> GGSGGSMPPPADIVKVAIEWPGAYPKLMEIDQKKPLSAIIKEVCDGWSLANHEYFALQHADSSNFYITEKNRNEIKNGTILRLTTSPAQNAQQLHERIQSSSMDAKLEALKDLASLSRDVTFAQEFINLDGISLLTQMVESGTERYQKLQKIMKPCFGDMLSFTLTAFVELMDHGIVSWDTFSVAFIKKIASFVNKSAIDISILQRSLAILESMVLNSHDLYQKVAQEITIGQLIPHLQGSDQEIQTYTIAVINALFLKAPDERRQEMANIL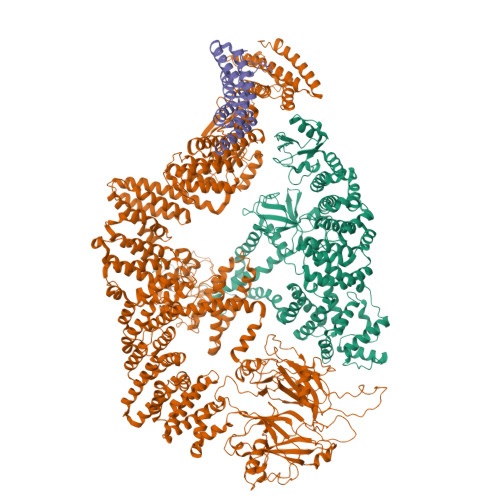AQKQLRSIILTHVIRAQRAINNEMAHQLYVLQVLTFNLLEDRMMTKMDPQDQAQRDIIFELRRIAFDAESEPNNSSGSMEKRKSMYTRDYKKLGFINHVNPAMDFTQTPPGMLALDNMLYFAKHHQDAYIRIVLENSSREDKHECPFGRSSIELTKMLCEILKVGELPSETCNDFHPMFFTHDRSFEEFFCICIQLLNKTWKEMRATSEDFNKVMQVVKEQVMRALTTKPSSLDQFKSKLQNLSYTEILKIRQSERMNQEDFQSRPILELKEKIQPEILELIKQQRLNRLVEGTCFRKLNARRRQDKFWYCRLSPNHKVLHYGDLEESPQGEVPHDSLQDKLPVADIKAVVTGKDCPHMKEKGALKQNKEVLELAFSILYDSNCQLNFIAPDKHEYCIWTDGLNALLGKDMMSDLTRNDLDTLLSMEIKLRLLDLENIQIPDAPPPIPKEPSNYDFVYDCN;>GGSGGSMARWIPTKRQKYGVAIYNYNASQDVELSLQIGDTVHILEMYEGWYRGYTLQNKSKKGIFPETYIHLKEATVEDLGQHETVIPGELPLVQELTSTLREWAVIWRKLYVNNKLTLFRQLQQMTYSLIEWRSQILSGTLPKDELAELKKKVTAKIDHGNRMLGLDLVVRDDNGNILDPDETSTIALFKAHEVASKRIEEKIQEEKSILQNLDLRGQSIFSTIHTYGLYVNFKNFVCNIGEDAELFMALYDPDQSTFISENYLIRWGSNGMPKEIEKLNNLQAVFTDLSSMDLIRPRVSLVCQIVRVGHMELKEGKKHTCGLRRPFGVAVMDITDIIHGKVDDEEKQHFIPFQQIAMETYIRQRQLIMSPLITSHVIGENEPLTSVLNKVIAAKEVNHKGQGLWVSLKLLPGDLTQVQKNFSHLVDRSTAIARKMGFPEIILPGDVRNDIYVTLIHGEFDKGKKKTPKNVEVTMSVHDEEGKLLEKAIHPGAGYEGISEYKSVVYYQVKQPCWYETVKVSIAIEEVTRCHIRFTFRHRSSQETRDKSERAFGVAFVKLMNPDGTTLQDGRHDLVVYKGDNKKMEDAKFYLTLPGTKMEMEEKELQASKNLVTFTPSKDSTKDSFQIATLICSTKLTQNVDLLGLLNWRSNSQNIKHNLKKLMEVDGGEIVKFLQDTLDALFNIMMEMSDSETYDFLVFDALVFIISLIGDIKFQHFNPVLETYIYKHFSATLAYVKLSKVLNFYVANADDSSKTELLFAALKALKYLFRFIIQSRVLYLRFYGQSKDGDEFNNSIRQLFLAFNMLMDRPLEEAVKIKGAALKYLPSIINDVKLVFDPVELSVLFCKFIQSIPDNQLVRQKLNCMTKIVESTLFRQSECREVLLPLLTDQLSGQLDDNSNKPDHEASSQLLSNILEVLDRKDVGATAVHIQLIMERLLRRINRTVIGMNRQSPHIGSFVACMIALLQQMDDSHYSHYISTFKTRQDIIDFLMETFIMFKDLIGKNVYAKDWMVMNMTQNRVFLRAINQFAEVLTRFFMDQASFELQLWNNYFHLAVAFLTHESLQLETFSQAKRNKIVKKYGDMRKEIGFRIRDMWYNLGPHKIKFIPSMVGPILEVTLTPEVELRKATIPIFFDMMQCEFNFSGNGNFHMFENELITKLDQEVEGGRGDEQYKVLLEKLLLEHCRKHKYLSSSGEVFALLVSSLLENLLDYRTIIMQDESKENRMSCTVNVLNFYKEKKREDIYIRYLYKLRDLHRDCENYTEAAYTLLLHAELLQWSDKPCVPHLLQRDSYYVYTQQELKEKLYQEIISYFDKGKMWEKAIKLSKELAETYESKVFDYEGLGNLLKKRASFYENIIKAMRPQPEYFAVGYYGQGFPSFLRNKIFIYRGKEYERREDFSLRLLTQFPNAEKMTSTTPPGEDIKSSPKQYMQCFTVKPVMSLPPSYKDKPVPEQILNYYRANEVQQFRYSRPFRKGEKDPDNEFATMWIERTTYTTAYTFPGILKWFEVKQISTEEISPLENAIETMELTNERISNCVQQHAWDRSLSVHPLSMLLSGIVDPAVMGGFSNYEKAFFTEKYLQEHPEDQEKVELLKRLIALQMPLLTEGIRIHGEKLTEQLKPLHERLSSCFRELKEKVEKHYGVITL[2x]hexyl 2-O-(6-deoxy-alpha-L-galactopyranosyl)-beta-D-galactopyranoside | C18 H34 O10 | 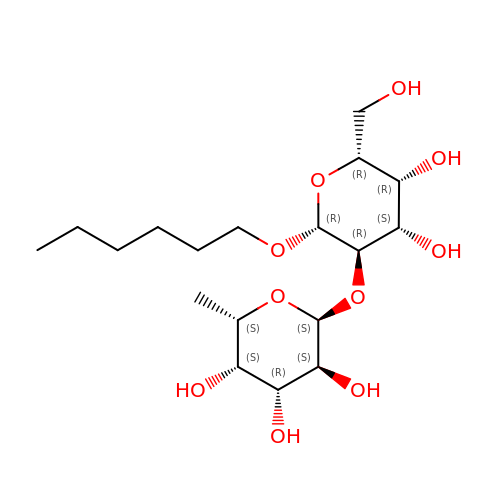FTONAEAQJAJCLK-LYVNYESWSA-N> AMADLEQKVLEMEASTYDGVFIWKISDFPRKRQEAVAGRIPAIFSPAFYTSRYGYKMCLRIYLNGDGTGRGTHLSLFFVVMKGPNDALLRWPFNQKVTLMLLDQNNREHVIDAFRPDVTSSSFQRPVNDMNIASGCPLFCPVSKMEAKNSYVRDDAIFIKAIV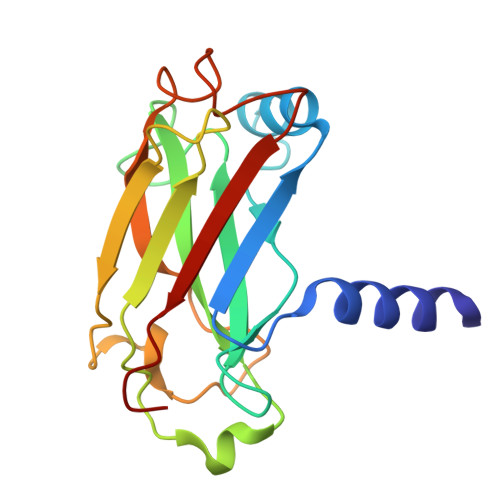DLTGL> LFNPEEFMPLDPTQEPIFPPELLRLKDVPPKQLRFEGERVTWIQASTLKELLDLKAQHPEAKLVVGNTEIGIEMKFKNQLFPMIICPAWIPELNAVEHGPEGISFGAACALSSVEKTLLEAVAKLPTQKTEVFRGVLEQLRWFAGKQVKSVASLGGNIITASPISDLNPVFMASGTKLTIVSRGTRRTVPMDHTFFPSYRKTLL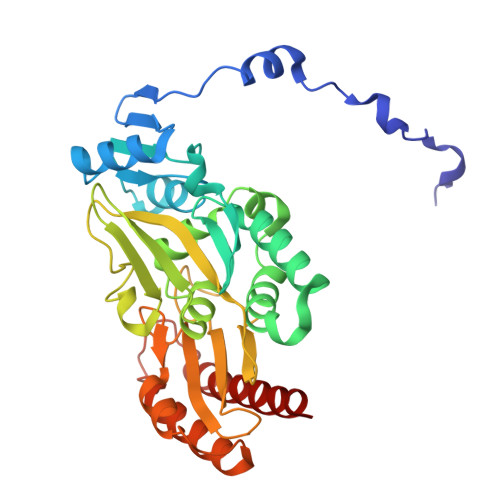GPEEILLSIEIPYSREDEFFSAFKQASRREDDIAKVTCGMRVLFQPGSMQVKELALCYGGMADRTISALKTTQKQLSKFWNEKLLQDVCAGLAEELSLSPDAPGGMIEFRRTLTLSFFFKFYLTVLKKLG>MRFLKRKKSLSAGMLLALAVGSAASIPSAYSNDDVLKLTENPKNWAAPGKDYANTRHSPLKQINTQNVKGLHMAWSFSTGVLRGHEGQPLVIGDRMYVVTPYPNIVWALDISKGNSYEVLWKYAPRQDDKAVSTACCDTVNRGASYADGKIVFNTLDGYVVCLDANTGKELWKTKFADVNKGETSTPAPIIVKDKVVTGYGGDEFGARGRFAAFDLNSGKMVWQAYSNGPDSDVLLGPDFNSKHPEYGQAGQDLGVKTYPDEEWKRGGGCAWGWYSYDPKLDLIYYNTGNPGLWSPSYRTE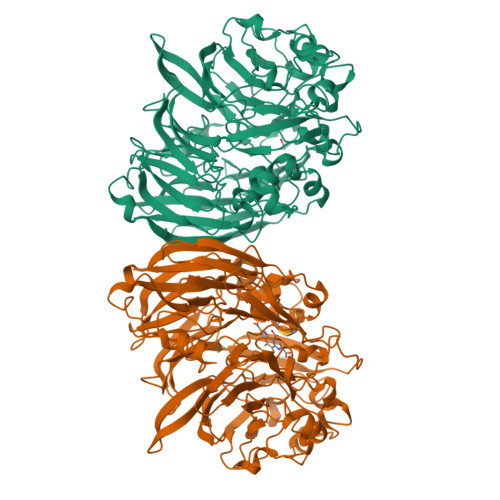AKTHEEANEPWKWDNKWSMTIFARKPDTGEAVWGYQMTPFDQWDYDGINEDVLVDITVDGSKKPCLVHFDRNGFCYVLNRTDGTIIRANKFVTVNWAEKIDMKTGRPVKVKEHSPFEVGKAVQAYPSAMGGKDQQPVAVDPKEPNVFYAPTNNWGMTLEPMERAHTNQGSVYVFANVLMKPEKPGVMGRFKAFDVITGKARWDIPERFPTWSGALVTDGGLAFYGTLDGWFKAVDRKTGKVLWQQKLGSGIIGNPISYEVGGKQYISVLSGIGGWIGLPVTAGLDPADPYGALGVSGMAAENGFYNIPMGGTLYTFCVQ[2x]> WVPHELNERQMERRKNTCEILLSRYKRKSFLHRIVTGDEKWIFFVNPKRKKSYVDPGQPATSTARPNRFGKKTMLCVWWDQSGVIYYELLKPGETVNAARYQQQLINLNRALQRKRPEYQKRQHRVIFLHDNAPSHTARAVRDTLETLNWEVLPHAAYSPDLAPSDYHLFASMGHALAEQRFDSYESVKKWLDEWFAAKDDEFYWRGIHKLPERWEKC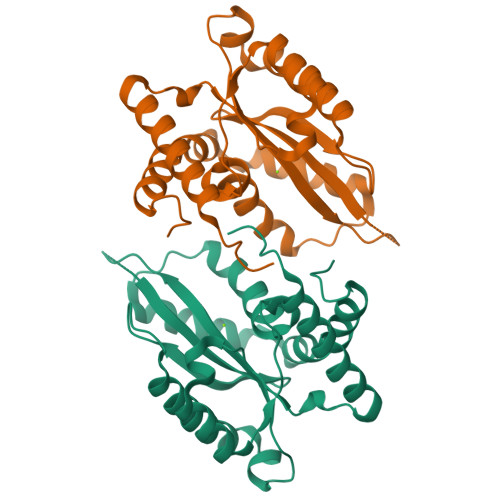VASDGKYFE4,7-DIMETHYL-[1,10]PHENANTHROLINE 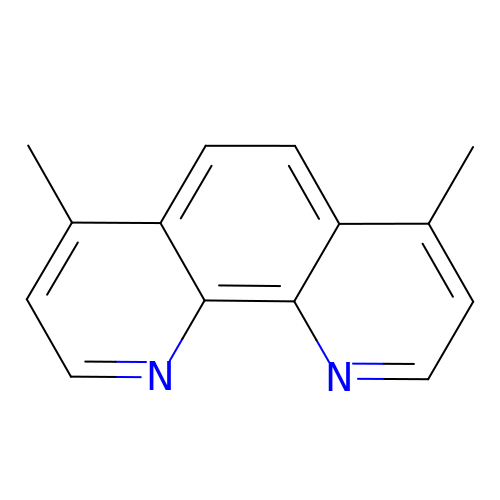| C14 H12 N2 | JIVLDFFWTQYGSR-UHFFFAOYSA-N> TGRPEWIWLALGTALMGLGTLYFLVKGMGVSDPDAKKFYAITTLVPAIAFTMYLSMLLGYGLTMVPFGGEQNPIYWARYADWLFTTPLLLLDLALLVDADQGTILALVGADGIMIGTGLVGALTKVYSYRFVWWAISTAAMLYILYVLFFGFTSKAESMRPEVASTFKVLRNVTVVLWSAYPVVWLIGSEGAGIVPLNIQTLLFMVLDVSAKVGFGLILLRS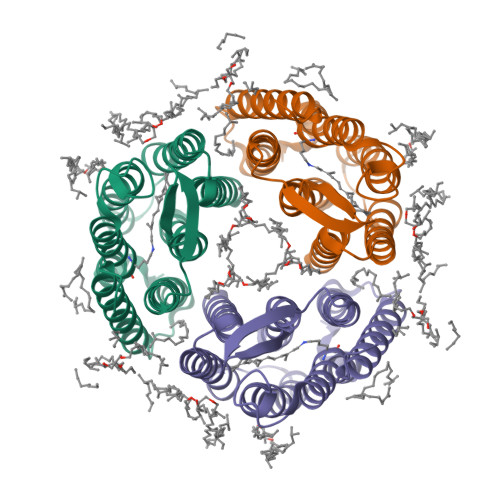RAIFG4-azanyl-6-[[(1~{S})-1-(3-methyl-5-oxidanylidene-6-phenyl-[1,3]thiazolo[3,2-a]pyridin-7-yl)ethyl]amino]pyrimidine-5-carbonitrile 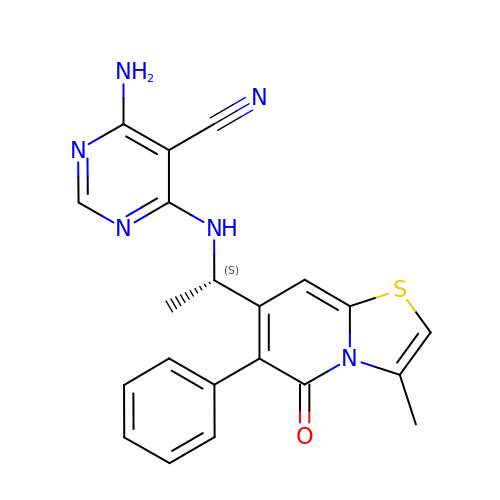| C21 H18 N6 O S | XLCBQUCCOPILIO-ZDUSSCGKSA-N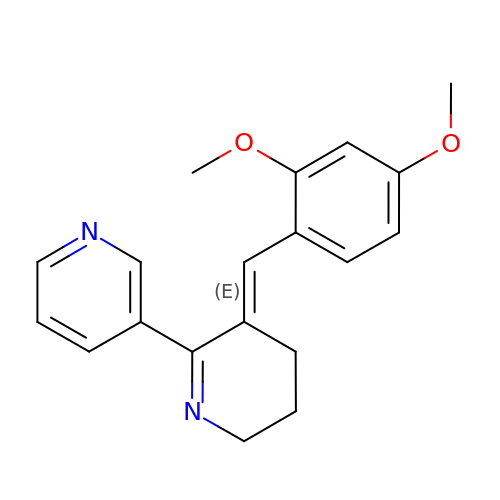(3E)-3-[(2,4-DIMETHOXYPHENYL)METHYLIDENE]-3,4,5,6-TETRAHYDRO-2,3'-BIPYRIDINE | C19 H20 N2 O2 | RPYWXZCFYPVCNQ-RVDMUPIBSA-N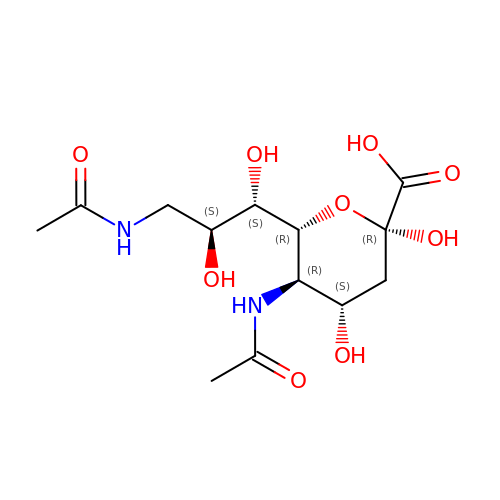(6R)-5-acetamido-6-[(1S,2S)-3-acetamido-1,2-dihydroxypropyl]-3,5-dideoxy-beta-L-threo-hex-2-ulopyranosonic acid | C13 H22 N2 O9 | VOVFDZJABRGWTQ-IAGKUOAJSA-N>[3x]ATAAEIAALPRQKVELVDPPFVHAHSQVAEGGPKVVEFTMVIEEKKIVIDDAGTEVHAMAFNGTVPGPLMVVHQDDYLELTLINPETNTLMHNINFHAATGALGGGGLTEINPGEKTILRFKATKPGVFVYHCAPPGMVPWHVVSGMNGAIMVLPREGLHDGKGKALTYDK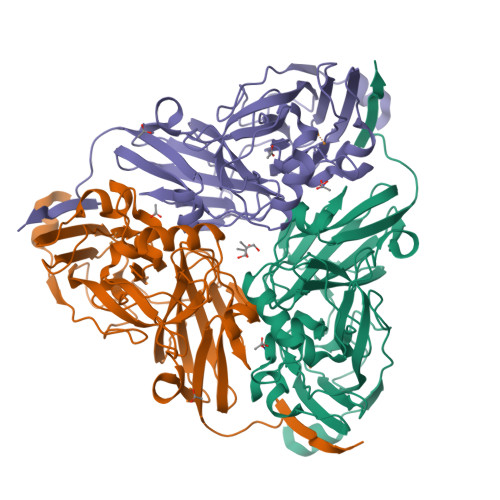IYYVGEQDFYVPRDENGKYKKYEAPGDAYEDTVKVMRTLTPTHVVFNGAVGALTGDKAMTAAVGEKVLIVHSQANRDTRPHLIGGHGDYVWATGKFNTPPDVDQETWFIPGGAAGAAFYTFQQPGIYAYVNHNLIEAFELGAAAHFKVTGEWNDDLMTSVLAPSGTIEGR> MSFFHGVTVTNVDIGARTIALPASSVIGLCDVFTPGAQASAKPNVPVLLTSKKDAAAAFGIGSSIYLACEAIYNRAQAVIVAVGVETAETPEAQASAVIGGISAAGERTGLQALLDGKSRFNAQPRLLVAPGHSAQQAVATAMDGLAEKLRAIAILDGPNSTDEAAVAYAKNFGSK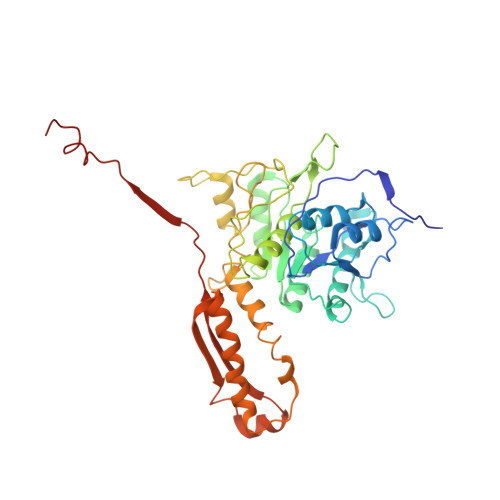RLFMVDPGVQVWDSATNAARNAPASAYAAGLFAWTDAEYGFWSSPSNKEIKGVTGTSRPVEFLDGDETCRANLLNNANIATIIRDDGYRLWGNRTLSSDSKWAFVTRVRTMDLVMDAILAGHKWAVDRGITKTYVKDVTEGLRAFMRDLKNQGAVINFEVYADPDLNSASQLAQGKVYWNIRFTDVPPAENPNFRVEVTDQWLTEVLDVA(6-benzyl-1-benzofuran-3-yl)acetic acid | C17 H14 O3 | 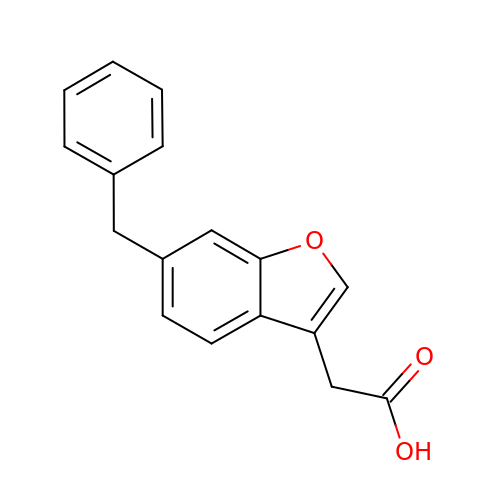NANLKTVMZIVCBJ-UHFFFAOYSA-N> NVIQDLYLRELKDT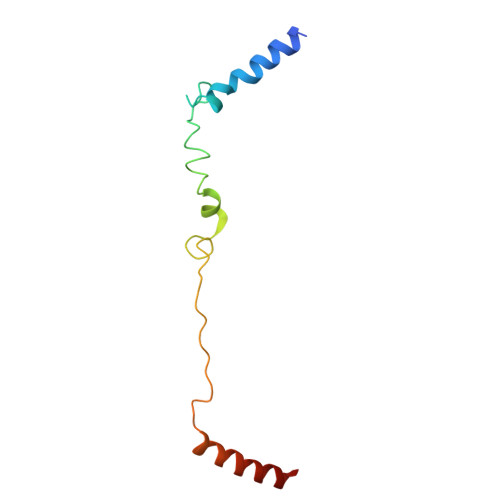KLAPSTLQDAEGNVKPWNPPQKPNLPELELQGPEALKAYTEQNVETAHVAKESEEGESEPIEEDWLVLDDAEETKESH>[2x]MATSLNTIDIQGDILVGMHKQKQLFYFFAINDPATFKTHLASDIAPVVASVTQLSNVATQPLVALNIAFSNTGLLALGVTDNLGDSLFANGQAKDATSFKESTSSWVPQFAGTGIHGVIILASDTTDLIDQQVASIESTFGSSISKLSSLSASIRPGNEAGHEMFGFLDG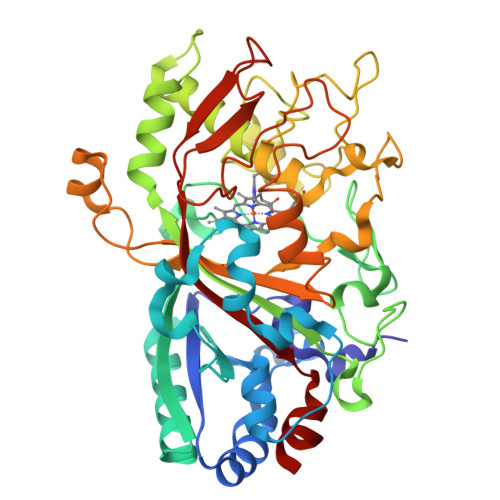IAQPAINGFNTPLPGQNIVDAGVIITGATNDPITRPSWAVGGSFLAFRQLEQLVPEFNKYLLDNAPAGSGSLQARADLLGARMVGRWKSGAPIDLTPTADDPALGADAQRNNNFTYSHAGFDLGSDQSHCPFSAHIRKTRPRADLGGSLTPPNLSAGANSIMRSGIPYGPEVTSAESASNTTTQERGLAFVAYQAQLSQGFHFLQQTSADNANFPPGKTPATVGLDPIIGQNNGQPRVVNGLLPSNSSASLSIPQFVVSHGGEYFFSPPISAIGGRLSA>[2x]GVFTFEDEITSTVPPAKLYNAMKDADSITPKIIDDVKSVEIVEGNGGPGTIKKLTIVEDGETKFILHKVESIDEANYAYNYSVVGGVALPPTAEKITFETKLVEGPNGGSIGKLTLKYHTKG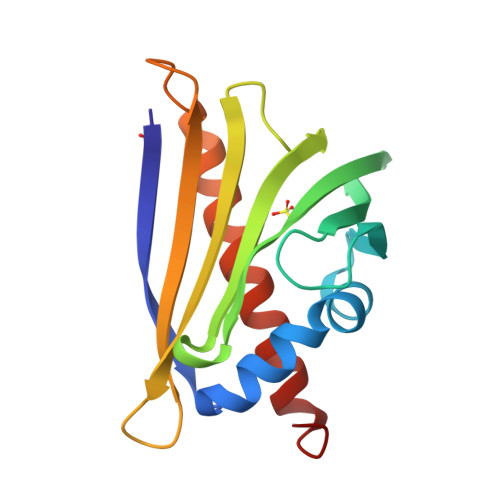DAKPDEEELKKGKAKGEGLFRAIEGYVLANPTQY>[16x]MTYAVAFRLERGLVFAADTRTNAGVDNIAQYKKLQLWRQPGERVFVLLSAGNLAATQAVVS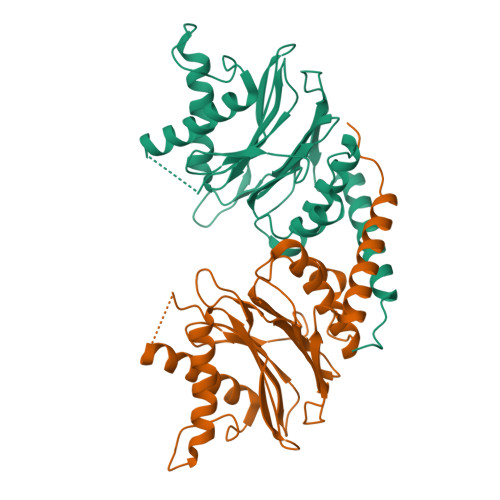LINEHLSQETDDEVTTLFTAPNMYRAARVVGDAVREARSIDGAALEASKLGFNTNFIFGGQIKGERPRLFQIYPEGNFIEATDDTPFFQIGEHKYGKPILDRVARSDMRLGEAAKLMLLSFDSTLRSNLSVGMPIDLVIYERDTFDVTREKRISADDEYFRNLSNAWSDALRQAFSKIEEFDV>MPSYLSPGVYVEEVASGSRPIEGVGTSVAAFVGLAPTGPLNEPTLVTNWTQYVAAFGDFTGGYYLAHSVYGFFNNGGSAAYVVRVGGSAEDAAADGSVNGAAAPAAVTGSTAKALPAAEPKQLGTFAVTATAAGQSGPLTVEVADPEGEGPAERFKLIVKDGDKPVETFDVSAKKGNRSYVVTQVKERSKLITVTEAAPSAQLVRPENQSLTLPAPPSAAPAVPAGQAESAHPGPAQYLGDSSDRTGFGGLEAIDEISMVAVPDLMAAYQRGAIDLEAVKAVQLGLIAHCELMGDRVAIIDPPPNQNARQIRVWRQETAGYDSKYAALYYPWIKSFDPATGQSRLVPPSGHVAGIWARNDSERGVHKAPANEVVRGAVDLELQITRGEQDLLNPIGVNCIRSFPGRGIRVWGARTLSSDPAWRYLNIRRYFNYLEESILIGTQWVVFEPNDHNLWARIRRNVSAFLVNEWRNGALFGQSPDQAYYVKCDEETNPPESVDLGRVVCEIGIAPVKPAEFVIFRLAQFSSGGG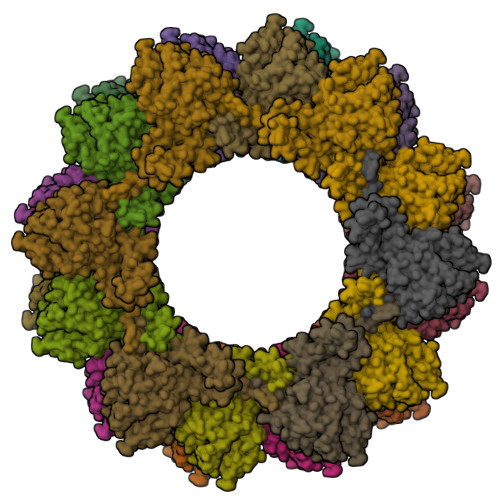ELDE[24x]> GSHMANLDRTDDLVYLNVMELVRAVLE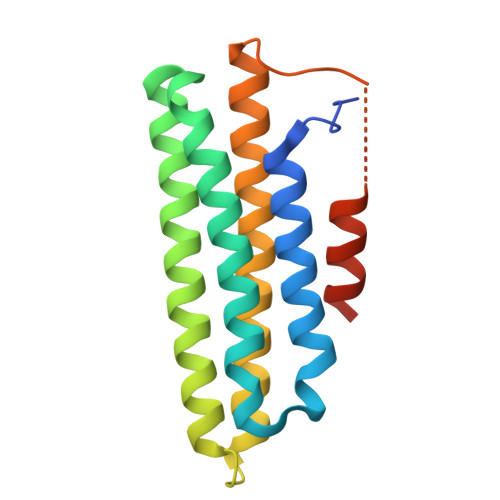LKNELSQLPPEGYVVVVKNVGLTLRKLIGSVDDLLPSLPSSSRTEIEGTQKLLNKDLAELINKMRLAQQNAVTSLSEEAKRQMLTASHTLAVDAKNLLDAVDQAKVLANLAHGGSGGGGGMEELDALLEELERSTLQDSD> UGGAAGAAAUCGAAGAAGAUGAAGAACGCGAAGAAC;>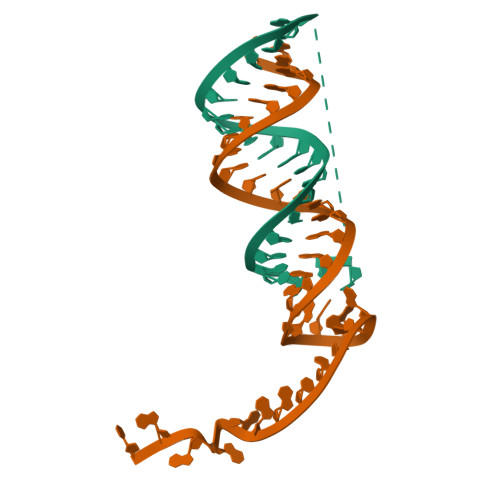 AUCUUCUUCGAUUUCUUCCAGUUCUUCGCGUUCUUC>[2x]NYKKPKLLYCSNGGHFLRILPDGTVDGTRDRSDQHIQLQLSAESAGEVYIKGTETGQYLAMDTEGLLYGSQTPNE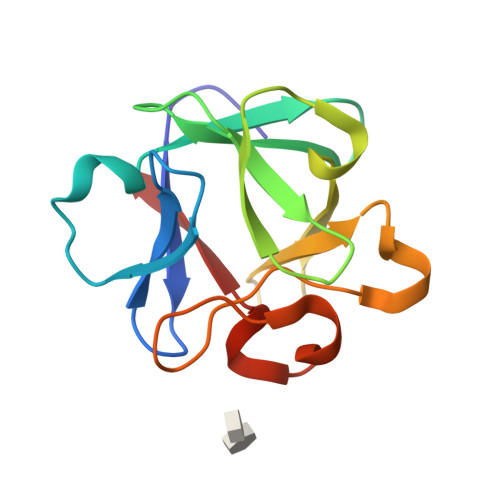ECLFLERLEENHYNTYTSKKHAEKNWFVGLKKNGSCKRGPRTHYGQKAILFLPLPVS> MLSERAHHRSLLTGREREIFQLLVRDYSTKDI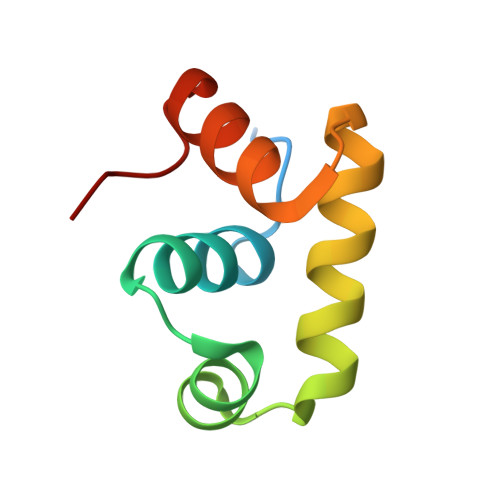SIQLKISEKTVRNHISNTIQKLGVSGRSQAILELLRLGELSLD3-[(1E)-3-oxo-3-({4-[1-(phenylcarbonyl)piperidin-4-yl]butyl}amino)prop-1-en-1-yl]-1-beta-D-ribofuranosylpyridinium 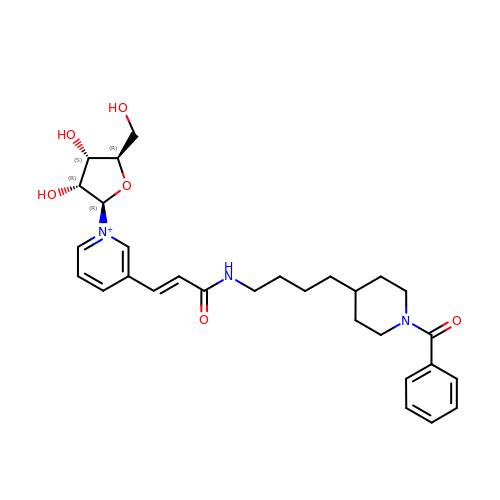| C29 H38 N3 O6 | NQSRPUVKZPKDIV-NNOPKNNOSA-O>[2x]GAMSLGKRLKEARQKAGYTQKEAAEKLNIGNNNLSNYERDYRDPDTDTLLKLSNLYNVSTDYLLGK

ICEBs1 is regulated by the ImmR/ImmA tandem, which are a transcriptional repressor that constitutively blocks transcription and a metallopeptidase that acts as anti-repressor and inactivates ImmR by proteolytic cleavage. Regulation of ICEBs1 is exerted by the Int integrase, the ImmR transcriptional repressor, and the ImmA anti-repressor metallopeptidase, which are counter-transcribed from the PimmR promoter of the transposon. In contrast, if the global DNA damage response is launched or if potential recipient cells lacking the transposon are nearby, ImmA inactivates ImmR by proteolytic cleavage, which unleashes ICEBs1 expression and promotes transposon transfer. We here report the production and purification of 127-residue ImmR from ICEBs1 and the crystal structure of its DNA-binding domain.

After successive rounds of model building and refinement, the final model comprised residues M1–K64 of molecules A and B, plus respective N-terminal alanines (A0) from the purification tag, and 167 solvent molecules. Remarkably, the final Fourier map did not show relevant density beyond K64 of either protomer, which would be compatible with the full-length molecule set up for crystallisation being proteolytically processed after this lysine by a trypsin-like contaminant. The protein is a compact almost spherical pentahelical bundle (α1–α5) cohered by a central hydrophobic core, in which the N- and the C-terminal helices are nearly antiparallel, so that the chain termini are adjacent. Helices α2–α4 form a flap that folds back onto the two terminal helices. Following the nomenclature of HTHGBB-DBDs26, helices α2 and α3 would correspond to the “positioning helix” and the “recognition helix” of the HTH-motif engaged in double-stranded DNA recognition. The two protomers in the asymmetric unit (a.u.) are related by a dyad, which gives rise to an interface of 573 Å2 (ΔiG = − 2.1 kcal/mol; ΔiG P-value = 0.42427). The main participating residues are L3, D41, T44, L47, L48, S51, N52, T58, D59, L62, and K64, which are provided by helices α4 and α5 plus the linker preceding α4. Finally, the experimental structure is in very good agreement with the predicted dimer. Accordingly, the DNA major groove would be contacted through the recognition helices, and flanking helices α3 and α4 would play a supportive role. Putative residues engaged in binding would encompass T17–E20, N29–N31, S33–Y35, R37, and Y39–D43 of either protomer.>MSEKKNIYPNKEGSPVEFTLDVIGGKWKGILFYHMIDGKKRFNEFRRICPSITQRMLTLQLRELEADGIVHREVYHQVPPKVEYSLTEFGRTL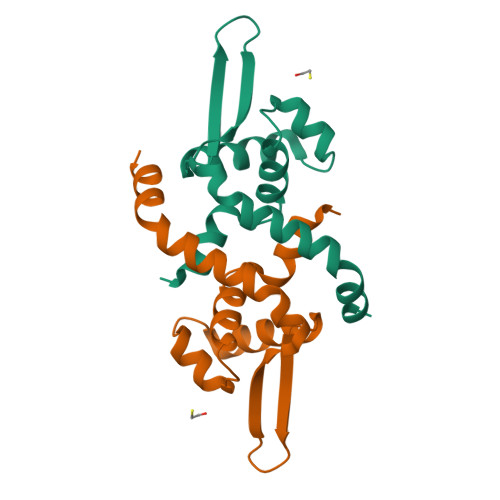EPIVLQMKEWGESNRDVLESYRSNGLVKDQQKHHHHHH[4x]>[5x]MEFWGIEVKSGKPVTVTPEEGILIHVSQASLGECKNKK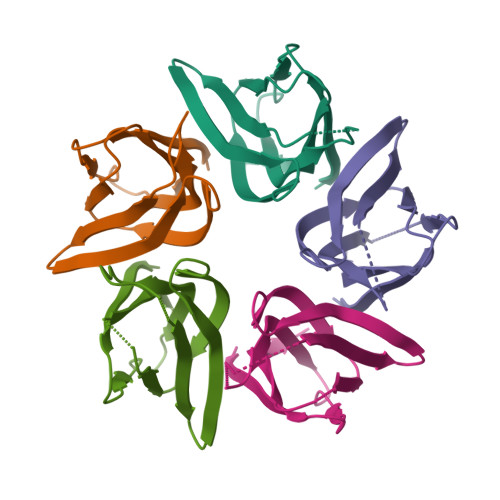GEFVPLHVKVGNQNLVLGTLSTENIPQLFCDLVFDKEFELSHTWGKGSVYFVGYKTPN5-ethyl-2-(3-methyl-1,2,3-triazol-4-yl)-1~{H}-benzimidazole 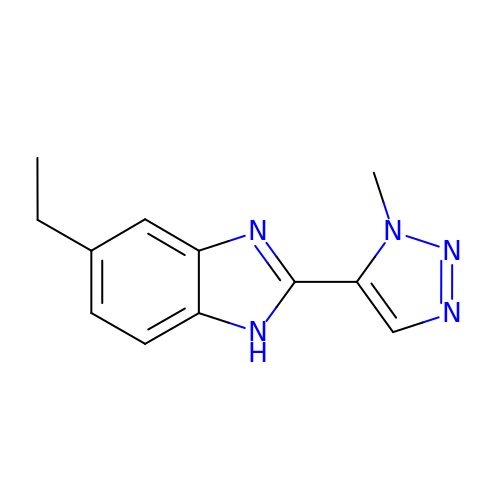| C12 H13 N5 | ODOFHRIEFOAOCH-UHFFFAOYSA-N> ETGRNLPKQLTQATQVAWSGPPPGFAKCPGGQVVILGFAMHLNFKEPGTDNFRIISCPPGREKCDGVGTASSETDEGRIYILCGEEPINEIQQVVAESPAHAGASVLEASCPDETVVVGGFGISVRGGSDGLDSFSIESCTTGQTICTKAPTRGSEKNFLWMMCVDKQYPGLRELVNVAELGSHGNANKRAVNSDGNVDVKCPANSSIVLGYVMEAHTNMQFVRDKFLQCPENASECKMTGKGVDHGMLWLFDRHALFGWIICKTVNEGTKHHHHHH

Toxoplasma and Plasmodium are the parasitic agents of toxoplasmosis and malaria, respectively, and use perforin-like proteins (PLPs) to invade host organisms and complete their life cycles. Escape from the PV, and therefore from the infected cell, for subsequent rounds of infection has been shown to be dependent on the perforin-like protein TgPLP1 (T. gondii PLP). We report structures of the membrane attack complex/perforin (MACPF) and Apicomplexan PLP C-terminal β-pleated sheet (APCβ) domains of TgPLP1. The MACPF domain forms hexameric assemblies, with ring and helix geometries, and the APCβ domain has a novel β-prism fold joined to the MACPF domain by a short linker.

An expression construct representing the TgPLP1 APCβ (residues 810 to 1072) was crystallized in space group C2 with the crystals diffracting to 1.1 Å resolution. The crystal structure of the C-terminal APCβ domain reveals a novel β-prism fold for the signature domain of the ApiPLPs. Comparison of the repeats with one another indicates a root mean square deviation (RMSD) of 1.28 to 1.56 Å over their roughly 80 residues each arranged into six β-strands with four forming one face of a sandwich and two the other. The two sides of the 4 + 2 sandwich forming each repeat are linked together by two highly conserved disulfide bonds, which can be treated as a signature motif of this domain. Among the other notable features of the TgPLP1 APCβ is the presence of a long projecting loop at its base, which is tipped by a tryptophan and has additional sequence features that make it resemble the similar loops found at the base of the CTDs of perforin itself and the CDCs. To determine whether the orientation with the long loop down toward the membrane gives the correct interface for membrane binding, we used site-directed mutagenesis combined with liposome sedimentation assays. Complementary to our findings from MD simulations, we found that the wild-type protein had a preference for POPE and also for PIP3-containing membranes, but that binding is reduced by mutation of the extended tip (MLWL→AAAA), by mutation of positively charged residues to neutral ones on the bottom of the domain (K→A, R→A), and by mutation of a histidine in the loop to alanine. The MLWL→AAAA and Lys/Arg→Ala mutants had a greater effect on binding than the His→Ala mutation did, which indicates the primacy of charge-based and hydrophobic interactions for stable membrane association.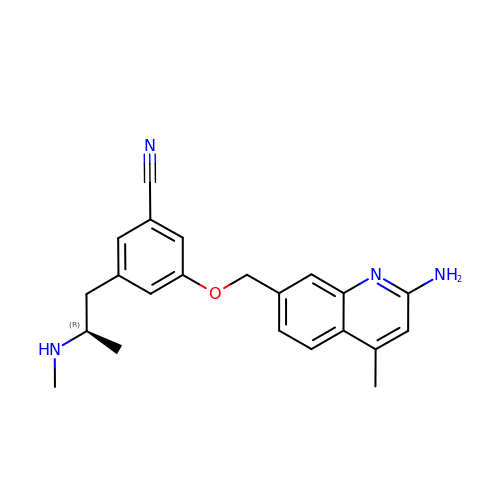3-[(2-amino-4-methylquinolin-7-yl)methoxy]-5-[(2R)-2-(methylamino)propyl]benzonitrile | C22 H24 N4 O | PUGNZMCPLRURSU-OAHLLOKOSA-N>EYNAPSEIKYIDVVNTYDLEEEASKVVPHGGFNYIAGASGDEWTKRANDRAWKHKLLYPRLAQDVEAPDTSTEILGHKIKAPFIMAPIAAHGLAHTTKEAGTARAVSEFGTIMSISAYSGATFEEISEGLNGGPRWFQIYMAKDDQQNRDILDEAKSDGATAIILTADSTVSGNRDRDVKNKFVYPFGMPIVQRYLRGTAEGMSLNNIYGASKQKISPRDIEEIAAHSGLPVFVKGIQHPEDADMAIKRGASGIWVSNHGARQLYEAPGSFDTLPAIAERVNKRVPIVFDSGVRRGEHVAKALASGADVVALGRPVLFGLALGGWQGAYS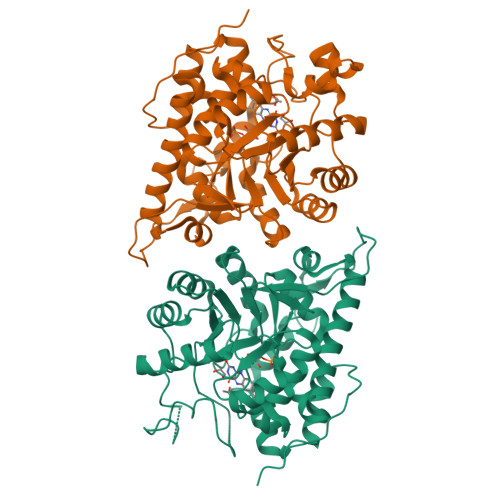VLDYFQKDLTRVMQLTGSQNVEDLKGLDLFDNPYGYEY[2x]> PLGSDSAKLIFINQINDCKDGQKLRFLGCVQSYKNGILRLIDGSSSVTCDVTVVLPDVSIQKHEWLNIVGRKRQDGIVDVLL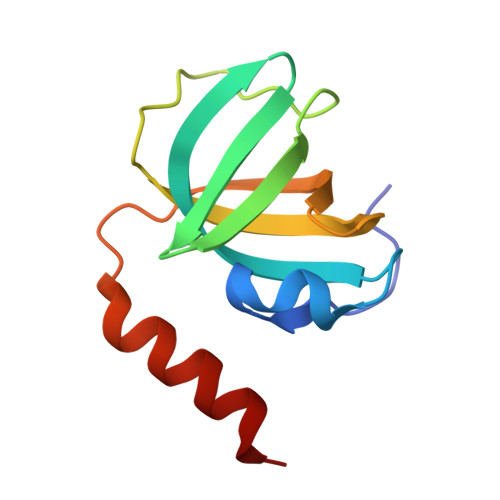IRSAVGINLPRYRQMVSERQKCD5-[2,4-bis(azanyl)pyrimidin-5-yl]oxy-2-methoxy-4-propan-2-yl-benzenesulfonamide 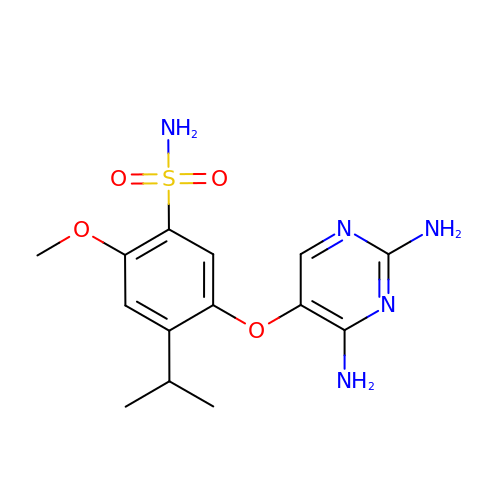| C14 H19 N5 O4 S | HLWURFKMDLAKOD-UHFFFAOYSA-N S-[2-(AMINOSULFONYL)ETHYL]-D-CYSTEINE | C5 H12 N2 O4 S2 | 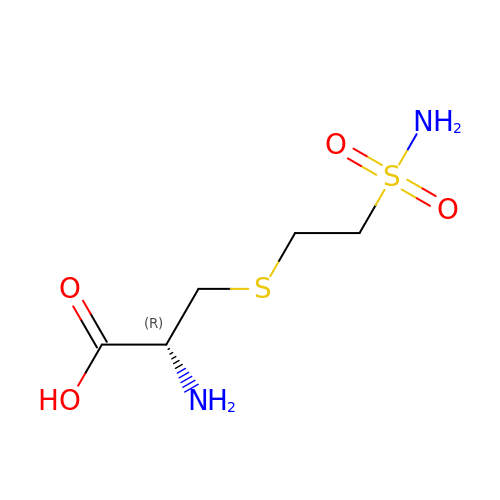ZRCBQBJBRHIRRG-BYPYZUCNSA-N>LGNFSQACYNSAIQGSVLTSTCIRTNGGYNTSSIDLNSVIENVDGSLKWQGSNFIETCRNTQLAGSSELAAECKTRAQQFVSTKINL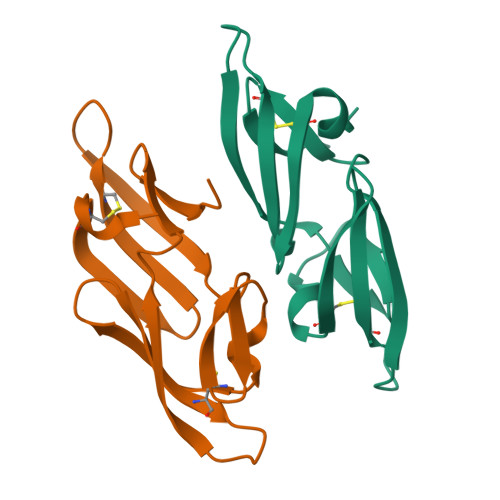DDHIAAIDGTLKYELEHHHHHH[2x]>[2x]GCUGACUAUGUGAUCUUAUUAAAAUUAGGUUAAAUUUCGA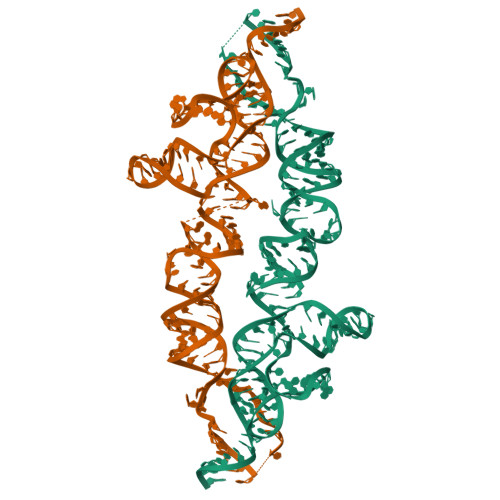GGUUAAAAAUAGUUUUAAUAUUGCUAUAGUCUUAGAGGUCUUGCGAAAGCUUACCACACAAGAUGGACCGGAGCGAAAGCUCCAAUAUCUAGUGUACCCUCG>MNTLSPRLRKAMNTAAWAHRHHVRKGGGIPYVSHLYSVMYLLASVTNDEDVLIAGLLHDTLEDVPEEYNSAQLEADFGPRVRELVEELTKQPLKSWKARADAYLLHLSAGASLEAVLISTADKLHNLMSILDDLEIHGEDLWQRFNAGKEQQIWWYSEVYQISLQRLGFNELNKQLGLCVEKLLKQSALEHHHHH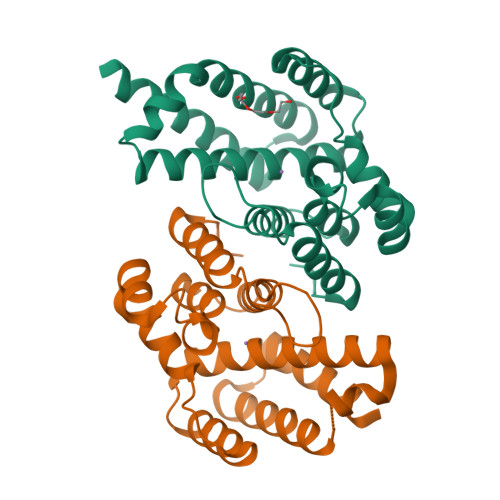H[2x]>[3x]DNDPLVVNTDKGRIRGITVDAPSGKKVDVWLGIPYAQPPVGPLRFRHPRPAEKWTGVLNTTTPPNSCVQIVDTVFGDFPGATMWNPNTPLSEDCLYINVVAPRPRPKNAAVMLWIFGGGFYSGTATLDVYDHRALASEENVIVVSLQYRVASLGFLFLGTPEAPGNAGLFDQNLALR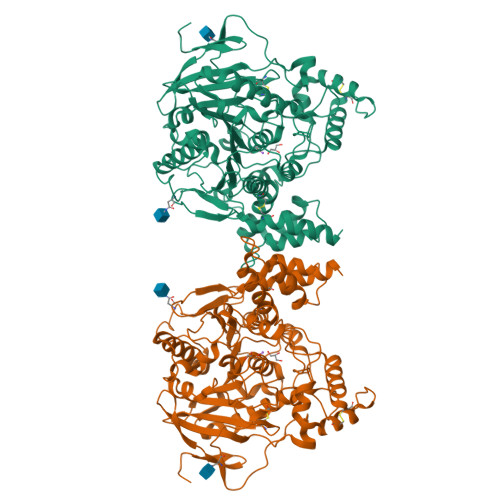WVRDNIHRFGGDPSRVTLFGESAGAVSVSLHLLSALSRDLFQRAILQSGSPTAPWALVSREEATLRALRLAEAVGCPHEPSKLSDAVECLRGKDPHVLVNNEWGTLGICEFPFVPVVDGAFLDETPQRSLASGRFKKTEILTGSNTEEGYYFIIYYLTELLRKEEGVTVTREEFLQAVRELNPYVNGAARQAIVFEYTDWTEPDNPNSNRDALDKMVGDYHFTCNVNEFAQRYAEEGNNVYMYLYTHRSKGNPWPRWTGVMHGDEINYVFGEPLNPTLGYTEDEKDFSRKIMRYWSNFAKTGNPNPNTASSEFPEWPKHTAHGRHYLELGLNTSFVGRGPRLRQCAFWKKYLPQLVAATSNLPGPAPPSEPCESSA> MGSERTCCPVNWVEHERSCYWFSRSGK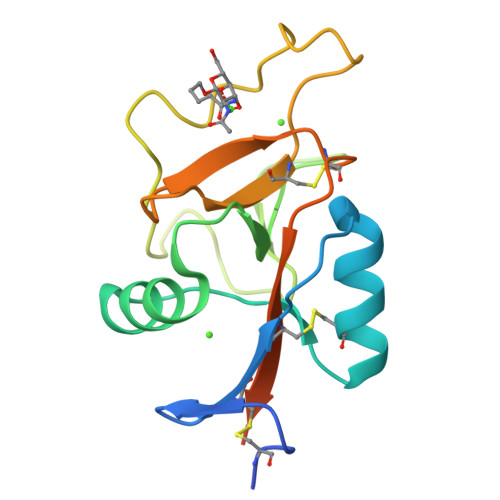AWADADNYCRLEDAHLVVVTSWEEQKFVQHHIGPVNTWMGLHDQNGPWKWVDGTDYETGFKNWRPEQPDDWYGHGLGGGEDCAHFTDDGRWNDDVCQRPYRWVCETELDKASQEPPLLGSHHHHHH> AKIGLFYGTQTGVTQTIAESIQQEFGGESIVDLNDIANADASDLNAYDYLIIGCPT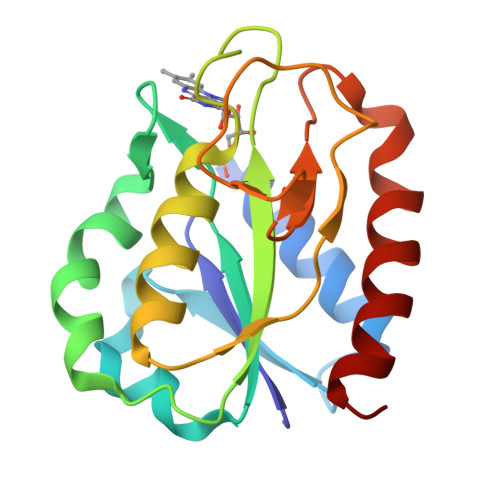WNVGELQSDWEGIYDDLDSVNFQGKKVAYFGAGNQVGYSDNFQDAMGILEEKISSLGSQTVGYWPIEGYDFNESKAVRNNQFVGLAIDEDNQPDLTKNRIKTWVSQLKSEFGL>VKSCKGRCFERTFSNCRCDAACVSLGNCCLDFQETCVEPTHIWTCNKFRCGEKRLSRFVCSCADDCKTHNDCCINYSSVCQDKKSWVEETCESIDTPECPAEFESPPTLLFSLDGFRAEYLHTWGGLLPVISKLKNCGTYTKNMRPMYPTKTFPNHYSIVTGLYPESHGIIDNK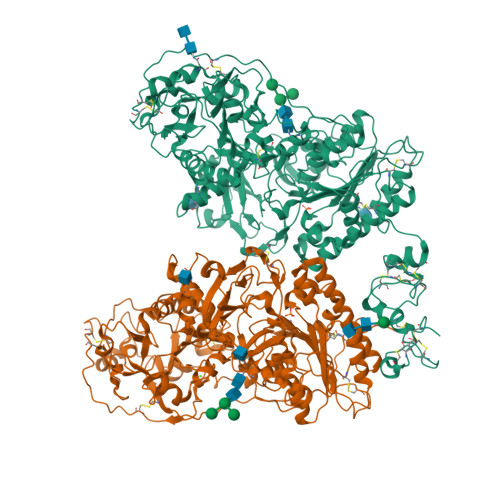MYDPKMNASFSLKSKEKFNPLWYKGQPIWVTANHQEVKSGTYFWPGSDVEIDGILPDIYKVYNGSVPFEERILAVLEWLQLPSHERPHFYTLYLEEPDSSGHSHGPVSSEVIKALQKVDRLVGMLMDGLKDLGLDKCLNLILISDHGMEQGSCKKYVYLNKYLGDVNNVKVVYGPAARLRPTDVPETYYSFNYEALAKNLSCREPNQHFRPYLKPFLPKRLHFAKSDRIEPLTFYLDPQWQLALNPSERKYCGSGFHGSDNLFSNMQALFIGYGPAFKHGAEVDSFENIEVYNLMCDLLGLIPAPNNGSHGSLNHLLKKPIYNPSHPKEEGFLSQCPIKSTSNDLGCTCDPWIVPIKDFEKQLNLTTEDVDDIYHMTVPYGRPRILLKQHHVCLLQQQQFLTGYSLDLLMPLWASYTFLRNDQFSRDDFSNCLYQDLRIPLSPVHKCSYYKSNSKLSYGFLTPPRLNRVSNHIYSEALLTSNIVPMYQSFQVIWHYLHDTLLQRYAHERNGINVVSGPVFDFDYDGRYDSLEILKQNSRVIRSQEILIPTHFFIVLTSCKQLSETPLECSALESSAYILPHRPDNIESCTHGKRESSWVEELLTLHRARVTDVELITGLSFYQDRQESVSELLRLKTHLPIFSQED[2x]>[2x]GHMPTPGTGSVPELQLVPFQLGHFPILQRWFATEKELVQWAGPALRHPLSLE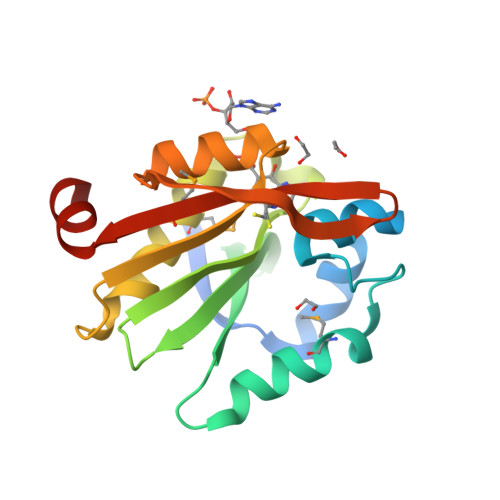QMHEDLAESRRRPPLRLLWSACRDDQVIGHCQLLFDRRNGVVRLARIVLAPSARGQGLGLPMLEALLAEAFADADIERVELNVYDWNAAARHLYRRAGFREEGLRRSATRVGRERWNVVLMGLLRQEWAAGGAGND N-{[3-(4-aminoquinazolin-7-yl)phenyl]sulfonyl}-L-threoninamide | C18 H19 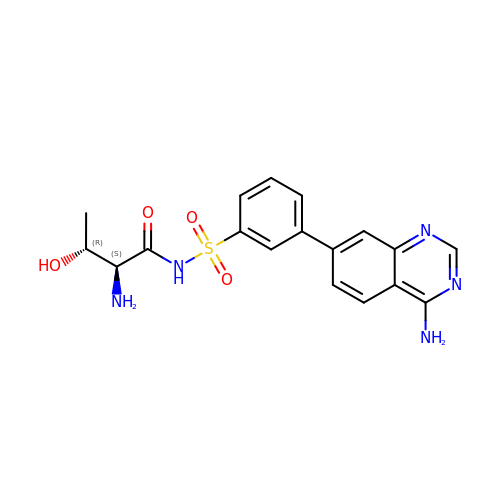N5 O4 S | QIPHQMPGDDKWIL-HWPZZCPQSA-N(2S)-3-(4-hydroxyphenyl)-2-isocyanopropanoic acid | C10 H9 N O3 | 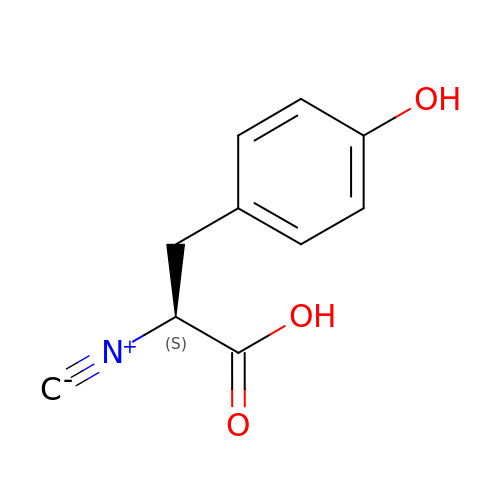YAVJAMZLLTZAJX-VIFPVBQESA-N> KPYNKIVSHLLVAEPEKIYAMPDPTVPDSDIKALTTLCDLADRELVVIIGWAKHIPGFSTLSLADQMSLLQSAWMEILILGVVYRSLSFEDELVYADDYIMDEDQSKLAGL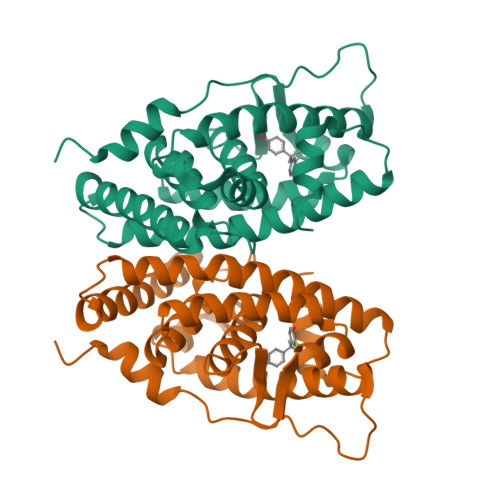LDLNNAILQLVKKYKSMKLEKEEFVTLKAIALANSDSMHIEDVEAVQKLQDVLHEALQDYEAGQHMEDPRRAGKMLMTLPLLRQTSTKAVQHFYNIKLEGKVPMHKLFLEMLEAKV6-[3-(dimethylamino)propyl]-4-methylpyridin-2-amine 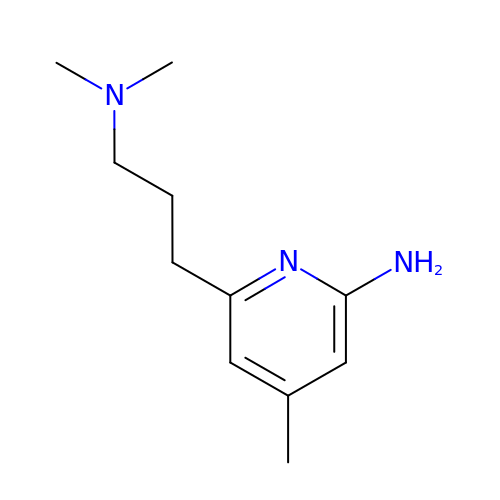| C11 H19 N3 | UOGCIQPLIAZGRO-UHFFFAOYSA-N> MKNNLPAFLFGTAMMVVMPPAAQAQSPATISLPQGGQFRLSISNTDPNMIFIPGDKVTAITAPGGMLADKRLTRAGGVLFTSVATRTFTIFVETARGQTFSVVATPVKGEGRVYRLMSAEPPSRPETRKWETAQAYEKLLISLNRAVLTGDIPDGYGEVKPLSDGIRLPGGFSVTPLKAWAGDQLRADRYELRNANTWGVALREQDF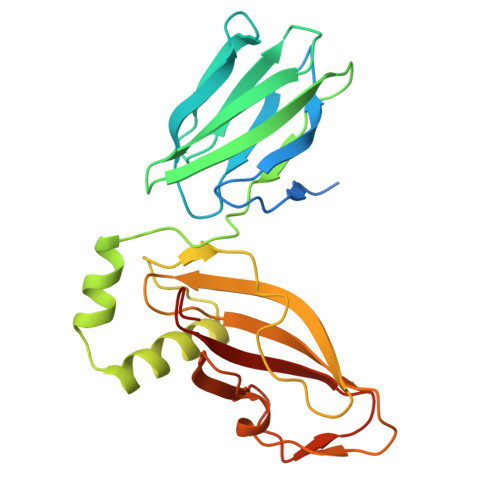WKPGVRAVMFDNNAQTLMGGGRMTVTVIRGNGEGEDGQR>[4x]MSSSENTLLDGKSENTIRFLTFNVNGIRTFFHYQPFSQMNQSLRSVFDFFRADIITFQQLKTEKLSISKWGRVDGFYSFISIPQTRKGYSGVGCWIRIPEKNHPLYHALQVVKAEEGITGYLTIKNGKHSAISYRNDVNQGIGGYDSLDPDLDEKSA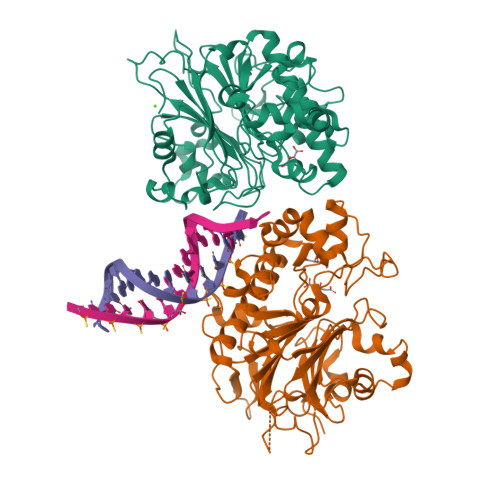LELDSEGRCVMVELACGIVIISVYCPANSNSSEEGEMFRLRFLKVLLRRVRNLDKIGKKIVLMGNVNVCRDLIDSADTLEQFSIPITDPMGGTKLEAQYRDKAIQFIINPDTPHRRIFNQILADSLLPDASKRGILIDTTRLIQTRNRLKMYTVWNMLKNLRPSNYGSRIDFILVSLKLERCIKAADILPDILGSDHCPVYSDLDILDDRIEPGTTQVPIPKFEARYKYNLRNHNVLEMFAKKDTNKESNENLYFQ>SNARVFNFAAGPATLPENVLLKAQADLYNWRGSGMSVMEMSHRGKEFLSIIQKAESDLRQLLEIPQEYSVLFLQGGATTQFAALPLNLCKSDDTVDFVVTGSWGDKAVKEAKKYCKTNVIWSGKSEKYTKVPSFEELEQTPDAKYLHICANETIHGVEFKDYPVPKNGFLVADMSSNFCSKPVDVSKFGVIYGGAQKNVGPSGVTIVIIRKDLIGNAQDITPVMLDYKIHDENSSLYNTPPCFGIYMCGLVFEDLLEQGGLKEVEKKNQRKADLLYNAIEESNGFFRCPVEKSVRSLMNVPFTLEKSELEAEFIKEAAKEKMVQLKGHRSVGGMRASIYNAMPLAGVEKLVAFMKDFQAKHA[4x]

PSATs are PLP-dependent enzymes that catalyze the second step of the phosphorylated pathway – reversible conversion of 3-PHP to PSer in a Glu-linked reaction. In this work, we describe a structure of the isoform 1 of chloroplastic PSAT from A. thaliana (At), which is further referred to in the manuscript as AtPSAT1. AtPSAT1 is a dimeric PLP-dependent AT that, similarly to other α-type ATs, binds the prosthetic group in the cavity within the large domain. The three crystal structures of AtPSAT1 present snapshots along the catalytic event showing PLP internal aldimine state, complex with PMP after the first half-reaction and PSer-PLP geminal diamine intermediate state.

The PLP prosthetic group creates a Schiff base (internal aldimine) between C4′ and Nζ of K265, the residue placed in the coil between β9 and β10. PLP is bound inside the active pocket with its pyridoxal ring π-stacked with W171 on the re-face of the cofactor. The protonated N1 of the pyridoxal ring is H-bonded to the carboxylate of D241. Another hydrogen bond is created between the hydroxyl group of PLP and T221. Phosphate of PLP creates a much more pronounced hydrogen bonding network with the protein. It includes direct H-bonds with backbone amides of A145 and T146, which, due to the placement at the N-terminal part of the α4 helix, possess an increased positive charge. Hydrogen bonds of PLP phosphate group also involve interactions with the side chain amide of Q264 and the hydroxyl group of T146. The phosphate also forms contacts with residues of the AtPSAT1 dimer mate, particularly hydrogen bonds with: the side chain amide of N306∗, the main chain amide of T307∗, and the side chain hydroxyl group of T307∗. Altogether, before the catalytic event, the PLP prosthetic group in AtPSAT1 structure presents a very conserved conformation in the internal aldimine state similar to that observed in other ATs, where C4′ atom of PLP is exposed to the entrance of the pocket. In case of the other two structures, the electron density maps are blurrier and with no meaningful signal for the side chain of R397, which indicates a flexibility of this region.> GPGKVVKFSYMWTINNFSFCREEMGEVIKSSTFSSGANDKLKWCLRVNPKGLDEESKDYLSLYLLLVSCPKSEVRAKFKFSILNAKGEETKAMESQRAYRFVQGKDWGFKKFIRRDFLLDEANGLLPDDKLTLFCEVSV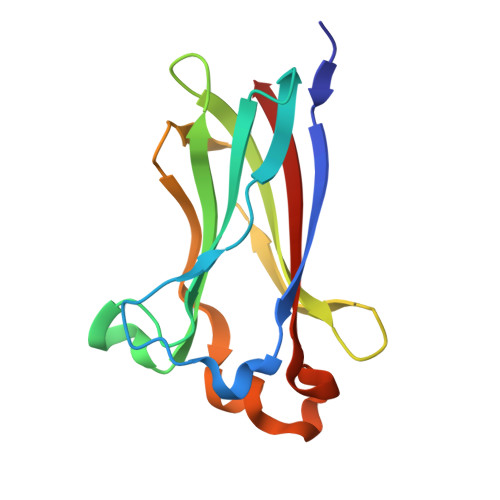VQD Oligopeptidase B (OPB, EC 3.4.21.83), an enzyme belonging to the prolyl oligopeptidase (PREP) family, has recently emerged as a virulence factor in T. brucei and other trypanosomes, and is a potential therapeutic target. OPB hydrolyses peptide substrates of up to 30 amino acid residues in length, after arginine or lysine with a preference for arginine and most efficiently after a pair of basic residues. The overall structure of TbOPB comprises the typical 2 domain α/β-hydrolase and β-propeller architecture that is present in all members of the PREP family structurally characterized to date. A short N-terminal segment (residues 1–87) and long C-terminal segment (residues 436–714) together form the α/β-hydrolase domain, whilst the region in between (residues 88–435) forms the β-propeller domain.

To this end, we have determined crystal structures of T. brucei OPB in the ligand-free open state and antipain-bound closed state. Crystal structures were determined in the ligand-free open state and inhibitor-bound closed state at resolution 2.4 and 2.85 Å, respectively. In this study, PISA identified two potential dimer interfaces present in the TbOPB open state structure, each involving ∼1000 Å2 of buried surface area. One interface involved contacts between the ãβ-hydrolase domain of one molecule with the β-propeller domain of the neighboring molecule, and included a disulfide bridge between Cys169 of each molecule. Without the closed state structure to compare with, it would have been easy to wrongfully assume that the lattice contact was the biological interface. With hindsight the lattice contact involving both domains and a disulfide bridge would impede the inter-domain flexibility needed to allow opening and closing of the enzyme during catalysis (discussed below), and therefore could not be the biological dimer interface. Fortuitous crystal contacts have presumably stabilized these more mobile regions in the TbOPB open state structure, resulting in complete electron density for these previously disordered regions. Domain separation pulls the propeller residue Glu172 out of and away from the active site. Whilst not directly involved in catalysis itself, this residue is responsible for fixing the crucial Arg650 in the appropriate catalytically active conformation in the closed state. In the open state, and in the absence of Glu172, Arg650 adopts a quite different position in the active site, binding instead to the catalytic triad Asp648, which in turn displaces the catalytic triad His683 to the surface of the molecule.

>[2x]MQTERGPIAAHRPHEVVFGKVEGEDRGANPMDPPRRRVDPLFWLRDDNRADPEVLAHLHLEKDYYEKRAVDIKDLAETIYQEHISHIEETDMSAPYVYDRFLYYTRDVKGLSYKLHCRVPAGKTPGEGEDEEIVLDENKLAEGKSFCVVGCVAPAPPEHALVAYSVDYCGDEVYSIRFVRDVVADKVEGTNGSVVWGPNAECFFYITKDASKRDNKVWRHIIGQPQSEDVCLYTDDDPLFSVGVGRSGDGKTLIICSMSSETSESHLLDLRKGVKHNTLEMVRPREKGVRYTVEMHGTDTLIVLTNKDKCVNGKVVLTKRSAPTDWGTVLIPHDDKVTIDDVAVFAKFAVLSGRRDGLTRVWTVRLGPDNLFSSATLKELHFDEPVFTAHVVCSQMKTYDASLLRLRYSSMTTPTVWYDEDVLSGERKVVKARKVGGGFESKNYVCRRELATAPDGTKVPISLVYDTSIDLKKPNPTMLYGYGSYGICIEPEFNSRFLPYVDRGMIYAIAHVRGGGEMGRTWYEVGGKYLTKRNTFMDFIACAEHLISSGLTTPAQLSCEGRSAGGLLVGAVLNMRPDLFHVALAGVPFVDVMTTMCDPSIPLTTGEWEEWGNPNEYKFFDYMNSYSPIDNVRAQDYPHLMIQAGLHDPRVAYWEPAKWASKLRELKTDSNEVLLKMDLESGHFSASDRYKYLRENAIQQAFVLKHLNVRQLLRK> MEIKEVDDRAELLRYTNNIPLLGKLVNHQPLWSTNPKLKSFSLEKISAPDQRRVQEALVVKDLLNVLIGLEGTYIRYFNDYEPSDPETPIEFKIAKKMDPSFKTFSRRIVRYGKQYMILTRAYEKWSDTSFGMVLQRFAYEIRRFLEDVYLKTLVERLERDFNKVPNFSIRELEQIINETEVNKQMELLYNIYEEIFREIEERRTNQSSQEDFNNFMDSMKNESSLHLRLMVAFDTTVYPVPKGGAILKIFQQKILENLGDRSSVMFLKKLLNNISQDYCTMLYEWLTQGILNDPYQEFMTYDDLEGKTDNIFDTRDRAWDTQYFIRKDVLLRDCDSEEDKNLLFKMLRTGILLKVVRASLQIPTIPSNSSDITIQEINDFADLMEGSNLELYVDKCYSRANEIFLKLFFQGYDLINVLKHLQQIFLGYQSGHNVLKFLTKNMGELTKHYRNDNNANYDKLLQNFELERQSENPNNLMRQLLMIQFDTETLPQVLSHYLQIYPEVPENNSANDDSDPLMHANNFKNMNAILFDELSKERTGAYHGSNLELYTPKSAIYHLKFDINIPYPLNIIISRTCMIKYQIILRYQLVLQYHSRLLDETWMDLNKTPSWKYRGYSHTVKRRIVRATRVLHAKMNHFIKTIMEYFNQNVIDKEVYSLEKCYRNPTLAVAIQNELEGGLTNIMTNRCLSDLIPLQLQIFDIVYKFCKFIKSMRAKLCQLDPVLYEKHKSGMMKTLNEGYRTNNGGQEDVGYQEDAALELIQKLIEYISNASSIFRKCLINFTQELSTEKFDFYDSSSVDAAGIERVLYSIVPPRSASASSQR;> MELEPTLFGIIEALAPQLLSQSHLQTFVSDVVNLLRSSTKSATQLGPLIDFYKLQSLDSPETTIMWHKIEKFLDALFGIQNTDDMVKYLSVFQSLLPSNYRAKIVQKSSGLNMENLANHEHLLSPVRAPSIYTEASFENMDRFSERRSMVSSPNRYVPSSTYSSVTLRQLSNPYYVNTIPEEDILKYVSYTLLATTSALFPFDHEQIQIPSKIPNFESGLLHLIFEAGLLYQSLGYKVEKFRMLNISPMKKALIIEISEELQNYTAFVNNLVSSGTVVSLKSLYREIYENIIRLRIYCRFTEHLEELSGDTFLIELNIFKSHGDLTIRKIATNLFNSMISLYYEYLMNWLTKGLLRATYGEFFIAENTDTNGTDDDFIYHIPIEFNQERVPAFIPKELAYKIFMIGKSYIFLEKYCKEVQWTNEFSKKYHVLYQSNSYRGISTNFFEIINDQYSEIVNHTNQILNQKFHYRDVVFALKNILLMGKSDFMDALIEKANDILATPSDSLPNYKLTRVLQEAVQLSSLRHLMNSPRNSSVINGLDARVLDLGHGSVGWDVFTLDYILYPPLSLVLNVNRPFGRKEYLRIFNFLWRFKKNNYFYQKEMLKSNDIIRSFKKIRGYNPLIRDIINKLSRISILRTQFQQFNSKMESYYLNCIIEENFKEMTRKLQRTENKSQNQFDLIRLNNGTIELNGILTPKAEVLTKSSSSKPQKHAIEKTLNIDELESVHNTFLTNILSHKLFATNTSEISVGDYSGQPYPTSLVLLLNSVYEFVKVYCNLNDIGYEIFIKMNLNDHEASNGLLGKFNTNLKEIVSQYKNFKDRLYIFRADLKNDGDEELFLLSKSLR;>MGGEIITLQAGQCGNHVGKFLWSQLAKEHAIGTDGLSQLPDSSTERDDDTKPFFR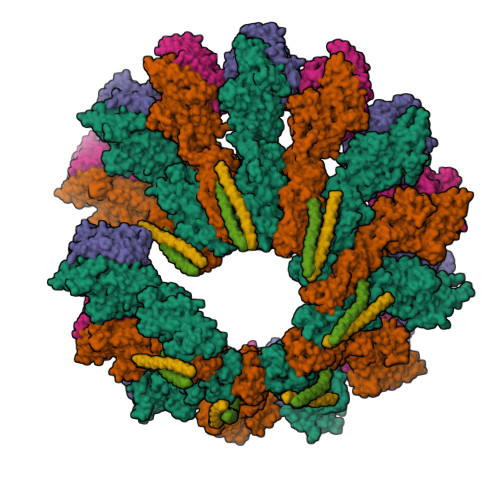ENCRNKFTPRAIMMDSEPSVIADVENTFRGFFDPRNTWVASDGASAGNSWANGYDIGTRNQDDILNKIDKEIDSTDNFEGFQLLHSVAGGTGSGLGSNLLEALCDRYPKKILTTYSVFPARSSEVVVQSYNTILALRRLIEDSDATVVFDNASLLNISGKVFRNPNIDLQHTNQLISTIISSVTNSIRFPSYMYSSMSSIYSTLIPSPELHFLSPSFTPFTSDYIHDDIAHKCHSSYDVMLDLLDPSNSLVSTAMNNPTYFNVYNTIIGNVEPRQISRAMTKLQQRIKFPSWSSSAMHVNIGRRSPYLPLQPNENEVSGMMLSNMSTVVNVFENACNTFDKVFAKGAFLNNYNVGDLFQSMQNVQDEFAESREVVQSLMEDYVAAEQDSYLDDVLVDDENMVGELEEDLDADGDHKLV[2x]> MAAVDIRDNLLGISWVDSSWIPILNSGSVLDYFSERSNPFYDRTCNNEVVKMQRLTLEHLNQMVGIEYILLHAQEPILFIIRKQQRQSPAQVIPLADYYIIAGVIYQAPDLGSVINSRVLTAVHGI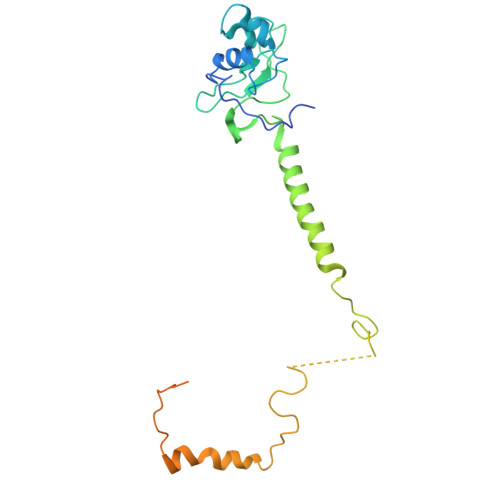QSAFDEAMSYCRYHPSKGYWWHFKDHEEQDKVRPKAKRKEEPSSIFQRQRVDALLLDLRQKFPPKFVQLKPGEKPVPVDQTKKEAEPIPETVKPEEKETTKNVQQTVSAKGPPEKRMRLQ>[3x]GPMGKPARKGAEWKRFLKNNWVLLSTVAAVVLGITTGVLVREHSNLSTLEKFYFAFPGEILMRMLKLIILPLIISSMITGVAALDSNVSGKIGLRAVVYYFATTLIAVILGIVLVVSIKPGVTQKVGEIARTGSTPEVSTVDAMLDLIRNMFPENLVQAAFQQYKTKREEVKPPSDPEMTMTEESFTAVMTTAISKTKTKEYKIVGMYSDGINVLGLIVFALVFGLVIGKMGEKGQILVDFFNALSDATMKIVQIIMWYMPLGILFLIAGCIIEVEDWEIFRKLGLYMATVLTGLAIHSIVILPLIYFIVVRKNPFRFAMGMAQALLTALMISSSSATLPVTFRCAEENNQVDKRITRFVLPVGATINMDGTALYEAVAAVFIAQLNDLDLGIGQIITISITATSASIGAAGVPQAGLVTMVIVLSAVGLPAEDVTLIIAVDCLLDRFRTMVNVLGDAFGTGIVEKLSKKELEQMDVSSEVNIVNPFALESTILDNEDSDTKKSYVNGGFAVDKSDTISFTQTSQF

Human excitatory amino acid transporters (EAATs) concentrate the neurotransmitter glutamate and aspartate in cells. By coupling the uptake of one substrate molecule to movements of five ions—symport of three sodium (Na+) ions and a proton and countertransport of one potassium (K+) ion—EAATs ensure that the cytoplasmic glutamate concentration is ~10 mM, which is required for neuronal functions, while the extracellular concentrations are as low as a few nM permitting rounds of synaptic signaling. EAATs are homotrimers composed of promoters that work independently. TMs 1, 2, 4, and 5 of each protomer comprise the scaffold domain mediating trimerization; TMs 3, 6, 7, and 8 and helical hairpins (HPs) 1 and 2 form the substrate-binding transport domain.

iOFS-K+ and iOFS-Apo imaged in the KCl and alkali-free NMDG buffers, respectively, have similar structures and feature well-resolved HP2s closed over the substrate-binding sites, although the hairpin conformations differ. What are the structural correlates distinguishing translocation-competent and translocation-incompetent states? iOFS-Apo is structurally similar to iOFS-K+ (RMSD of 0.52 Å for the transport domains); both feature apo configurations of the NMD and YE/DDR motifs. However, in translocation-incompetent iOFS-Apo and iOFS-Na+, HP2 residues coordinating K+ and Na2 and residues 414–417 at the start of the HP2b helix unwind and form an enlarged loop with an opening in the middle (states highlighted in pink), resembling an unzipped purse. The potassium binding to iOFS-Apo and glutamate to iOFS-Na+ zip HP2s, increasing their helicity and decreasing dynamics, as evidenced by the better-defined HP2 EM density of iOFS-K+ compared to iOFS-Apo. In contrast, deprotonated E374 of apo EAAT3 is engaged with R447 and cannot stabilize the helix, necessitating K+ binding to zip the hairpin. Comparing iOFS-Na+ to iOFS-Apo structures, we observed that sodium binding led to M367 in the NMD motif shifting into the binding pocket and R447 in the YE/DDR motif shifting out. Thus, in contrast to iOFS-Na+, iOFS-Apo cannot bind and translocate glutamate, preventing the dissipation of the glutamate gradient. In iOFS-Apo and iOFS-Na+, E374 is solvent-accessible through the unzipped HP2 and likely deprotonated with pKa-s of 6.5 and 7.1, respectively.(1~{S})-1-[(4-hydroxyphenyl)methyl]-6-methoxy-1,2,3,4-tetrahydroisoquinolin-7-ol 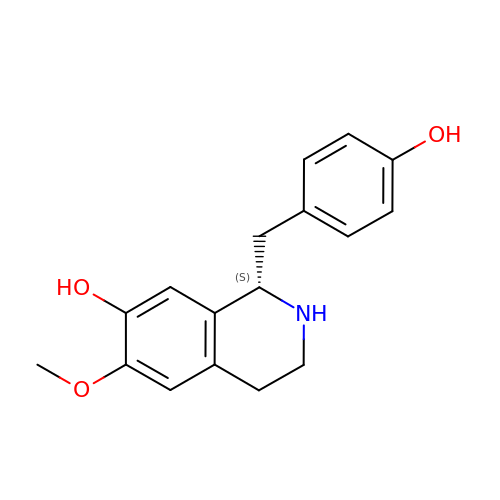| C17 H19 N O3 | LVVKXRQZSRUVPY-HNNXBMFYSA-N>HEEEDVICDGCNGPVVGTRYKCSVCPDYDLCSVCEGKGLHRGHTKLAFPSPFGHLSEGFS[4x]

Intriguingly, the autophagy adapter p62/SQSTM1/Sequestosome-1 was recently reported to recognize N-degrons, the N-end rule substrates of the well-characterized UPS, and where ultimately these substrates are delivered to ALS8,9. p62 is a key selective autophagy adapter that plays a role in the degradation of various cellular constituents such as misfolded proteins and their aggregates, malfunctioning organelles, and invading pathogens. Intriguingly, it was recently reported that the central ZZ-domain in p62 plays a critical role in the recognition of N-terminal arginylated BiP/GRP78 by the Arg-tRNA transferase ATE1. Here, we present the high resolution structures of the ZZ-domain of p62 in complex with 8 different N-degrons including type-1 and type-2, and subsequently identify key determinants involved in the unusual recognition.

Therefore, we determined the structure of the ZZ-domain in complex with a variety of N-degrons comprising three type-1 N-degrons and five type-2 N-degrons. As described for the R-BiP complex, two aspartic acid residues, Asp129 and Asp149, bind to the α-amino group, and Asp147 forms a hydrogen bond with the first peptide bond, which means that these interactions are conserved in all different N-terminal residues. However, the side chain of the N-terminal residue of the N-degron is recognized differently. The side chain of Asn132 which undergoes a conformational change plays a critical role in interacting with the first residue of the N-degron. The bipolar nature of the side chain atoms (O and N) of Asn132 allow for the recognition of positively charged type-1 substrates as well as type-2 substrates, and especially N-terminal tyrosine and tryptophan residues since they possess polar atoms in the side chain. The binding affinity between the ZZ-domain and other type-1 substrates with histidine or lysine residues at the primary position showed ca. a 10-fold reduction, although it was still significant.4-amino-N-(cyclohexylmethyl)-1,2,5-oxadiazole-3-carboxamide | C10 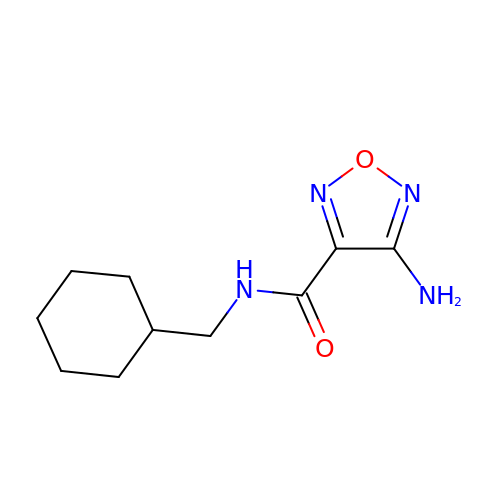H16 N4 O2 | LMUMGZXENBDFGR-UHFFFAOYSA-N>[2x]SNAMESPLGSDLARLVRIW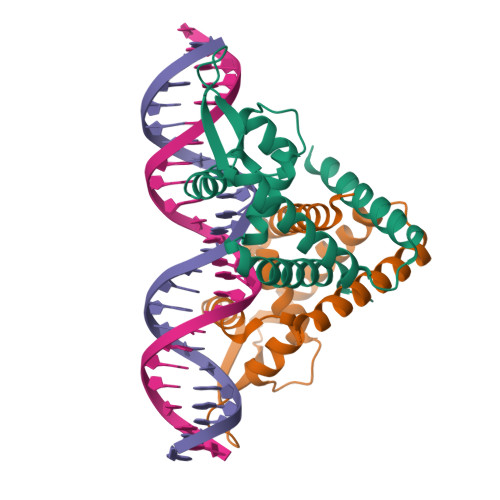RALIDHRLKPLELTQTHWVTLHNIHQLPPDQSQIQLAKAIGIEQPSLVRTLDQLEDKGLISRQTCASDRRAKRIKLTEKAEPLIAEMEEVIHKTRGEILAGISSEEIELLIKLIAKLEHNIMELHSHD>[2x]DTSGTVCLSALPPEATDTLNLIASDGP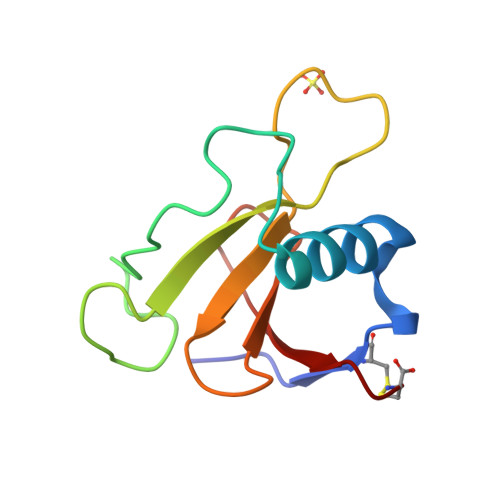FPYSQDGVVFQNRESVLPTQSYGYYHEYTVITPGARTRGTRRIITGEATQEDYYTGDHYATFSLIDQTC> MRTTKFLALALCLLASASALSANNSAPSNDWWDIPYPSQFDVKSLKTQSFISVKGNKFIDDKGKTFTFRGVNIADTGKLLSRNQWQKSLFEELANNWGVNTIRLPIHPVSWRKLGPDVYLGHIDEAVRWANDLGIYLILDWHSIGYLPTEQYQHPMYDTTIKETRDFWR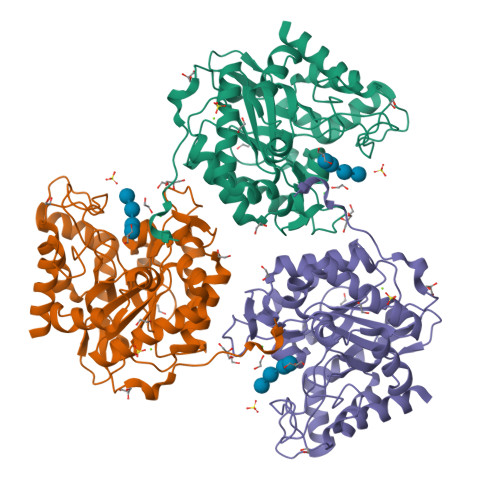RITFRYQNVPTVAVYELFNEPTTMGNTLGERNWAEWKTLNESLIDMIYASDKTVIPLVAGFNWAYDLSPIKKAPIEREGIAYAAHPYPQKAKPEVKNDKNFFKLWDEKWGFAADTYPVIATQLGWVQPDGYGAHIPVKDDGSYGPRIVKYMQKKGVSYTVWVFDPDWSPTMINDWDFTPSEQGAFFKQVMLEAKKR>MEASRRDFISIGIGALGAVGGLGALYALVRVMLEPSEIAALGAKTEIDVSKIQPMQVRVTSWKGKTLFAIRLPKDFKPEGYTLKKGALNSKGTTNYEILKGHDVFALVGVCTHLGCIPLWKPQGEGGINKPVFHCPCHGGLYTPYGDVIGGPPPRPLFIPPQKLEGNKLIVGVEGFVKELI[2x];>MGLIEKIVDWIDERAHVREIYRTQMVEYKVAKNLTFPYVFGILALVTFAIQIISGMVLILYYKPSIADAFDSATYSIMGEIPFGWLFRHIHATGANFFMAIVYLHMFTGIYYNAYKRPRELVWIVGWLIYFVLILTALSGYLLPWGQLSYWGFIVTTEIPGSLADAPILKPIFKAIAETIVLWMKGGYVVTDVTLGRVFGSHVLIYPLILLALVGIHLYLVRAAGISNPEGIEYDKKKNPDKFVPFHPYMTLKEGAYVMWYLAVFFFFVFFHISHFLPPENFEPANPLKTPAHIAPEWYLLGYYEVFRSIPSKFWGFVAFNALLLLLLLLPFLDFSPLKS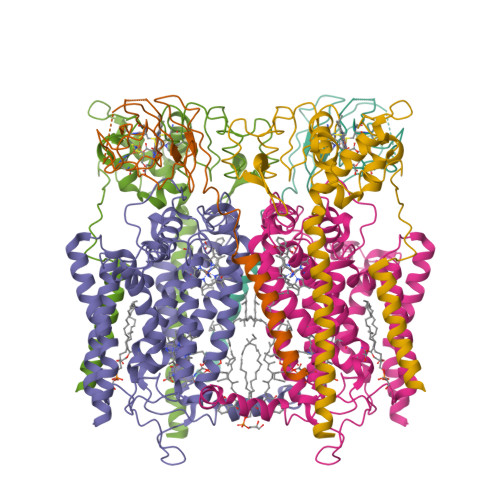ARRRPLFFVMFVIFMISSMALTILGTMPPTPQNAKLGLIFAALVFAFFISLPIISFIEYGWYKAKGGQQE[2x];>MNTWGLIKTIFFAGSTLVFFFLLWFYNPFKHVEHYEVDEEVKAIIDNPWKKTESGKTIAEEGRELFIASCSSCHSLRYDGIYIMSVAANPKWKNIEKTSGRPVYRFGTLYKDRFFVPKDVYEAFAHDDIQGLKASLGQVPPDLSSMYLARGEGYLYQFILNPQKVLPGTTMPQLFNPQFDPQAKEKVAKIVAYMKSVNTPPPKESAKRTVMGVIVIAYFIVMGLLLWKYRENLLKRLGYH[2x]Except for an N-terminal region, Prp3 is highly conserved from yeast to human and contains a C-terminal domain of unknown function (DUF1115; PFAM ID PF06544). Here, we showed that Prp3 orthologs contain a C-terminal U4/U6 di-snRNA binding region that encompasses a DUF1115 domain and a preceding peptide rich in basic residues. Our crystal structure and targeted mutational analyses demonstrate that the DUF1115 domain acts as a ssRNA-binding domain that specifically recognizes the first 10 nts of the U6 3′-overhang. Our results indicate how Prp3 functionally bridges U4/U6 and U5 in the tri-snRNP by Prp3-RNA interactions on one side and Prp3-protein interactions on the other.

We also determined the crystal structure of yPrp3DUF1115, lacking the preceding basic peptide, at 2.0 Å resolution. While the ordered parts of yPrp3CTF and yPrp3DUF1115 are very similar (RMSD of 0.48 Å for 131 common Cα atoms), the β3a/β3b hairpin in yPrp3DUF1115 is positioned closer to the globular part of the protein, showing that its relative positioning is indeed flexible. The lower apparent affinity estimated by EMSA is likely due to the presence of non-specific tRNA competitor in this assay. The yPrp3 DUF1115 domain (residues 325–469; yPrp3DUF1115) lacking the preceding basic peptide showed ca. twofold reduced affinity for yU4/U6stem II+13nt in EMSA (Kd,app 1.83 µM; Figure 1C, second gel and quantification) and a ca. 3.5-fold lower affinity in ITC (Kd 380 µM). In any case, these observations show that both the DUF1115 domain and the preceding basic peptide contribute to the RNA binding. Finally, Prp3CTF, but not the DUF1115 domain, inhibits Brr2-mediated U4/U6 unwinding, suggesting that the peptide stabilizes contacts between U4 and U6, presumably by binding the stem II duplex.

> GAMEAVNMNVEKPTVYHCKVFQFKNLQNPKIRFKLKMNSKELSLKGLCLRIRDDGPGIIIVVGNEKSCKFYENLVMKRIKWNEDFELHTNTGDIKMDMHNNSISKTWEGYLQDCKFKGWFMKVCNDQDSLLRTLGQFDSEHFYSPVQT>[8x]SSGLVPRGSHMSEMIYGIHAVQALLERAPERFQEVFILKGREDKRLLPLIHALESQGVVIQLANRQYLDEKSDGAVHQGIIARVKPGRQYQENDLPDLIASLDQPFLLILDGVTDPHNLGACLRSADAAGVHAVIVPKDRSAQLNATAKKVACGAAESVPLIRVTNLARTMRMLQEENIWIVGTAGEADHTLYQSKMTGRLALVMGAEGEGMRRLTREHCDELISIPMAGSVSSLNVSVATGI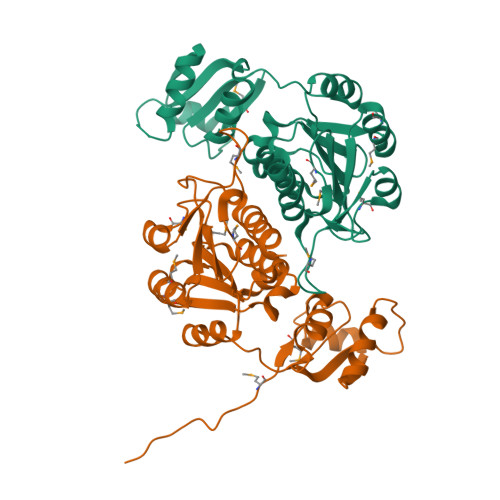CLFEAVRQRS>MGHHHHHHAENLYFQGADPMSKLSDSKSVFSKLSNKQIETIIQRYASPCFIIDENALLERARLFQQAILNQYQNSIAAYSVKTQSLNTIIQKFYEVGFIPEVVSSDEFEQIQKLQLCDKSIIFNGPYKNDASLIKALQLNAMINCDHFDEILRIAKIAKKLNITAKIGLRIADNKTPQNWSRFGFALTDQQNNSDIFTTIDKIQQIANIQLAGLHCHIGTNIRDISRFTAMAKNIAELAETILTKYKLTLEWIDLGGGLAGISPTLSDKRLQPYNPFDLELYAATIIAPLKEYLNKTNDKTKLIFELGRSLVDYSVALLTTIVGTREQNEDFQSLITDAGIHTIPTISTYRHPIYHLKTDSYHKKTLLLGPSCMQHDFLHDDIFLPKLEYGDKLLIDGVGAYNISRNNEFIHLKPSVILIDKNQQYQVLRVRQTHQ[4x]

The siderophore rhizoferrin (N1,N4-dicitrylputrescine) is produced in fungi and bacteria to scavenge iron. Francisella encodes a NIS synthetase FslA/FigA and an ornithine decarboxylase homolog FslC/FigC, required for rhizoferrin biosynthesis. Ornithine decarboxylase produces putrescine from ornithine, but we show here in vitro that FigA synthesizes N-citrylornithine, and FigC is an N-citrylornithine decarboxylase that together synthesize rhizoferrin without using putrescine. FigC belongs to a new subfamily of alanine racemase-fold PLP-dependent decarboxylases that are not involved in polyamine biosynthesis.

The X-ray crystal structure was solved to 2.1 Å resolution by single-wavelength anomalous diffraction using incorporated selenomethionine to phase the structure. Two functional dimers were found in the asymmetric unit (four monomers), and all four active sites showed good density for the cofactor PLP. FigC is composed of an N-terminal β/α-barrel domain and a C-terminal β-barrel domain, typical of the AR-fold PLP-dependent decarboxylases. The FigC active site is positioned at both the monomer domain interface and the dimer interface between the N-terminal β/α-barrel of one subunit and the β-barrel domain of the second. A Schiff base is formed between the PLP cofactor and the conserved catalytic lysine (K63 in FigC). Additional conserved residues with demonstrated roles in the catalytic cycle in these eukaryotic ODC enzymes are also observed to make key contacts with PLP in the FigC structure. These include E287, which interacts with the pyridine nitrogen of PLP to facilitate decarboxylation by stabilizing the carbanion intermediate; the glycine loop (G237–239) and R290, which form important backbone amide interactions with the phosphate of PLP contributing to tight binding; H198, which stacks against the PLP ring, and R151 positioned near the PLP hydroxyl. Additionally, C354, shown to function as a catalytic base in eukaryotic ODCs, is also conserved in FigC and contributes to the active site from across the dimer interface. First, the 310-helix has rotated out of the pocket to a greater extent than for any of the other structural homologs, and it projects two threonine residues (T327 and T330) and a tyrosine (Y331) into the pocket, all of which are likely to be in position to interact with the substrate based on the docked structure. The aspartate positioned next to the catalytic cysteine in L/ODC, ADC, and DAPDC, which interacts with the substrate side-chain amino group has been replaced by M355 in FigC. Finally the FigC structure has also evolved to use additional structural elements that are deeper in the pocket for substrate binding (e.g., R387), elements that were not needed for binding to the smaller substrates preferred by other enzymes in the family.>GSMDSSINCIEQTTEWSACSKSCGMGLSTRVTNRNLQCEMVKQTRLCMVRPCEQEPG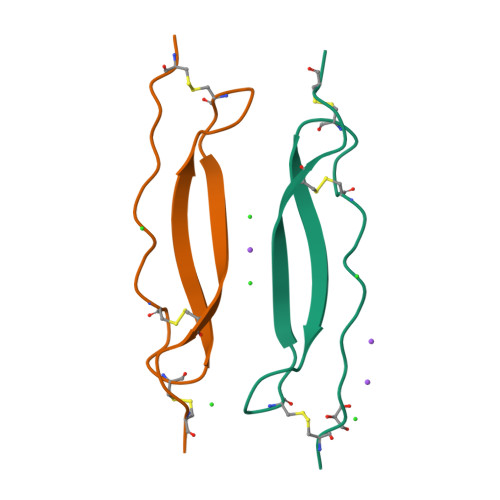E[2x]Herpesvirus-associated ubiquitin-specific protease (HAUSP, also known as USP7), a deubiquitylating enzyme of the ubiquitin-specific processing protease family, specifically deubiquitylates both p53 and MDM2, hence playing an important yet enigmatic role in the p53–MDM2 pathway. Here we demonstrate that both p53 and MDM2 specifically recognize the N-terminal tumor necrosis factor–receptor associated factor (TRAF)–like domain of HAUSP in a mutually exclusive manner. The crystal structures of the HAUSP TRAF-like domain in complex with p53 and MDM2 peptides, determined at 2.3-Å and 1.7-Å resolutions, respectively, reveal that the MDM2 peptide recognizes the same surface groove in HAUSP as that recognized by p53 but mediates more extensive interactions. Structure-based sequence alignment of the three HAUSP-binding peptides revealed a conserved four-residue binding motif with the consensus sequence of (Ø/E)-G-(Ø/G)-S, where Ø denotes a non-polar residue.

To facilitate formation of a stable p53–HAUSP complex, we generated a chimeric protein with the C-terminus of the HAUSP TRAF-like domain (residues 53–199) fused to ten amino acids corresponding to p53 residues 359–368. We reasoned that such design would ensure a 1:1 stoichiometry between HAUSP and the p53 peptide. The structure of the HAUSP TRAF-like domain bound to p53 (residues 359–368) was determined at 2.3-Å resolution by molecular replacement. Binding by the p53 peptide does not induce any significant conformational changes in HAUSP as shown by the structural comparison of the free and p53-bound TRAF-like domain. For example, Pro359 and Ser362 in the p53 peptide anchor its interaction with the HAUSP TRAF-like domain; missense mutation of Pro359 or Ser362 in p53 abolished its binding to HAUSP. Mutation of Trp165 and Phe167 in HAUSP, both involved in the hydrophobic pocket that accommodates Pro359 of p53, resulted in a complete loss of binding to p53 (unpublished data). Similarly, mutation of Asp164, which forms hydrogen bonds with S362 of p53, also significantly weakened the ability of HAUSP to bind to p53 (unpublished data). Two non-polar residues, Pro359 in p53 and Ala226 in MDM2, are positioned at the same site upon binding to HAUSP and make similar van der Waals contacts with a hydrophobic-surface pocket near the edge of β-sandwich in HAUSP. The residues following Pro359 in p53 and Ala226 in MDM2 are both glycines, which are very well superimposed and make conserved main-chain hydrogen bonds to Gly166 in the β7 strand of HAUSP. P3, a hydrophobic residue in MDM2 and EBNA1, stacks against a small hydrophobic-surface patch on HAUSP. This residue is Gly in p53, resulting in a loss of van der Waals interaction at the P3 position and consequently contributing to a relatively low binding affinity.

>[2x]GSHMNTAEEDMEDDTSWRSEATFQFTVERFSRLSESVLSPPCFVRNLPWKIMVMPRFYPDRPHQKSVGFFLQCNAESDSTSWSCHAQAVLKIINYRDDEKSFSRRISHLFFHKENDWGFSNFMAWSEVTDPEKGFIDDDKVTFEVFVQADAPGGSRAHSSH>[4x]LGSMSSIAISYGEGGSVFCGLKSDGSHLVVCYGSNSAILYGTPGHL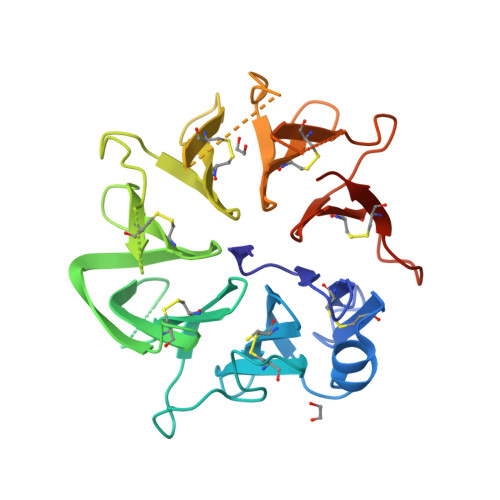QFIGLTGGDGFMCGLLMLSHQPYCWGNSAFIQMGVPQPMTKGAEYLEVSAGDYHLCGLRKPIVGRRKNSNIISSSLVDCWGYNMTRNFVFDKQLHSLSAGSEFNCALSSKDKSVFCWGDENSSQVISLIPKEKKFQKIAAGGYHVCGILDGLESRVLCWGKSLEFEEEVTGTSTEEKILDLPPKEPLLAVVGGKFYACGIKRYDHSAVCWGFFVNRSTPAPTGIGFYDLAAGNYFTCGVLTGTSMSPVCWGLGFPASIPLENLYFQ> TGSTGSTGSTGSQQKRAFEYEIRFYTGNDPLDVWDRYISWTEQNYPQGGKESNMSTLLERAVEALQGEKRYYSDPRFLNLWLKLGRLCNEPLDMYSYLHNQGIGVSLAQF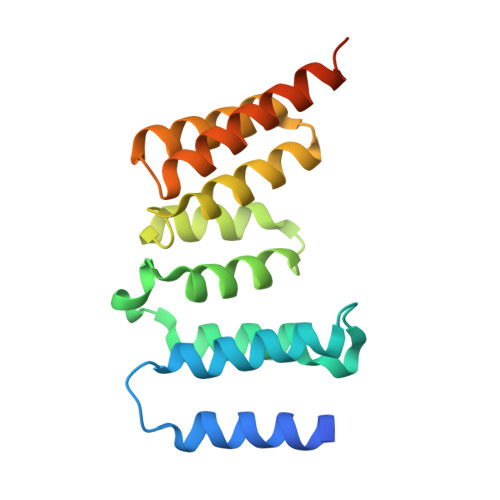YISWAEEYEARENFRKADAIFQEGIQQKAEPLERLQSQHRQFQARVSRQTLLALEKEEEEEVFESS> GSHMSNKEYRPTLAQLRTFVTIAECKHFGTAATKLSISQPSLSQALVALETGLGVQLIERSTRKVIVTPAGEKLLPFAKSTLDAAESFLSHAKGANGSLTGPLTVGIIPTAAPYILPSMLSIVDEEYPDLEPHIVEDQTKHLLALLRDGAIDVAMMALPSEAPGMKEIPLYDEDFIVVTASDHPFAGRQDLELSALEDLDLLLLDDGHCLHDQIVDLCRRGNINPISSTTAVTRASSLTTVMQLVVAGLGSTLVPISAIPWECTRPGLATANFNSDVTANRRIGLVYRSSSSRAEEFEQFALILQRAFQEAVALAASTGITLKQNV;> GSHMSNKEYRPTLAQLRTFVTIAECKHFGTAATKLSISQPSLSQALVALETGLGVQLIERSTRKVIVTPAGEKLLPFAKSTLDAAESFLSHAKGANGSLTGPLTVGIIPTAAPYILPSMLSIVDEEYPDLEPHIVEDQTKHLLALLRDGAIDVAMMALPSEAPGMKEIPLYDEDFIVVTASDHPFAGRQDLELSALEDLDLLLLDDGHCLHDQIVDLCRRGNINPISSTTAVTRASSLTTVMQLVVAGLGSTLVPISAIPWECTRPGLATANFNSDVTANRRIGLVYRSSSSRAEEFEQFALILQRAFQEAVALAASTG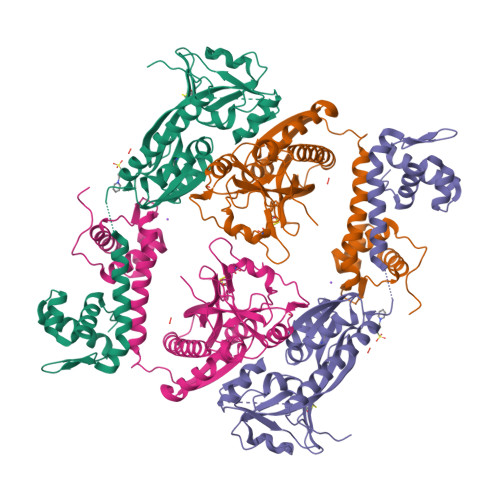ITLKQNVA>GHMPSSGKRRAPRRVYQIPQ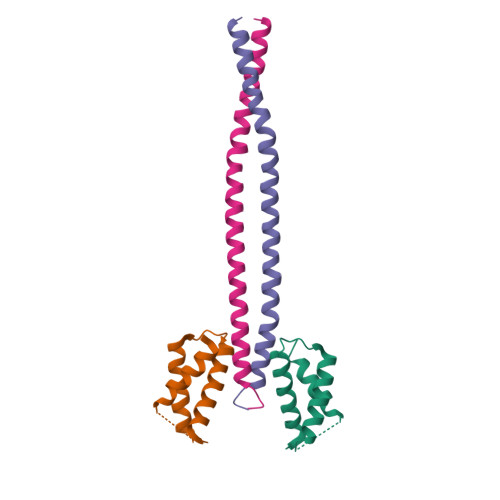RRRLQGKDPRWATMADLKMQAVKEICYEVALADFRHGRAEIEALAALKMRELCRTYGKPDGPGDAWRAVARDVWDTVGE[2x];>GHMEKLHEANNELQKKRAIIEDLEPRFNNSSLKIEELQEALRKKEEEMKQMEERYKKYLEKAKSVIRTLDPKQNQ[2x]> SMQEEDTFRELRIFLRNVTHRLAIDKRFRVFTKPVDPDEVPDYVTVIKQPMDLSSVISKIDLHKYLTVKDYLRDID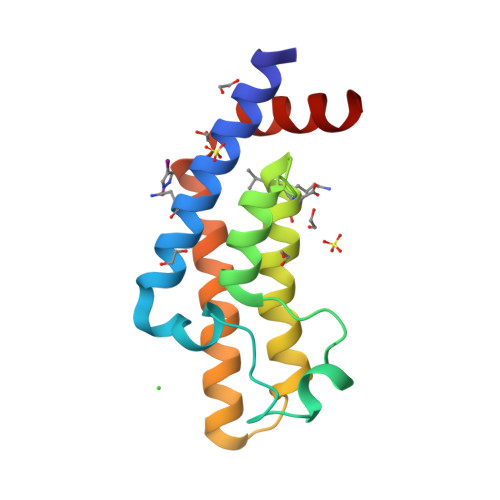LICSNALEYNPDRDPGDRLIRHRACALRDTAYAIIKEELDEDFEQLCEEIQESR> MLEQPYLDLAKKVLDEGHFKPDRTHTGTYSIFGHQMRFDLSKGFPLLTTKKVPFGLIKSELLWFLHGDTNIRFLLQHRNHIWDEWAFEKWVKSDEYHGPDMTDFGHRSQKDPEFAAVYHEEMAKFDDRVLHDDAFAAKYGDLGLVYGSQWRAWHTSKGDTIDQLGDVIEQIKTHPYSTRLIVSAWNPEDVPTMALPPCHTLYQFYVNDGKLSLQLYQRSADIF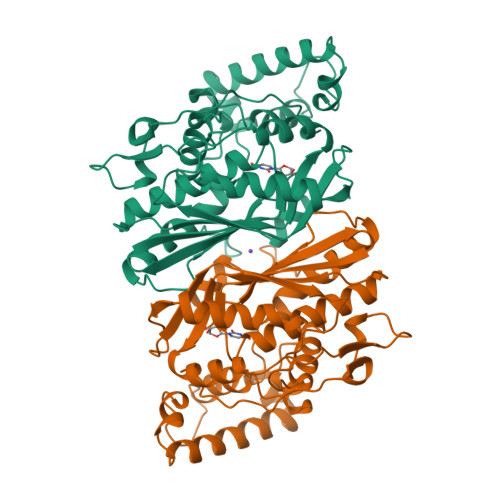LGVPFNIASYALLTHLVAHECGLEVGEFIHTFGDAHLYVNHLDQIKEQLSRTPRPAPTLQLNPDKHDIFDFDMKDIKLLNYDPYPAIKAPVAV> QNTVSHVSAACLFSEALHGIPFGVKVLKALAAANVSDASK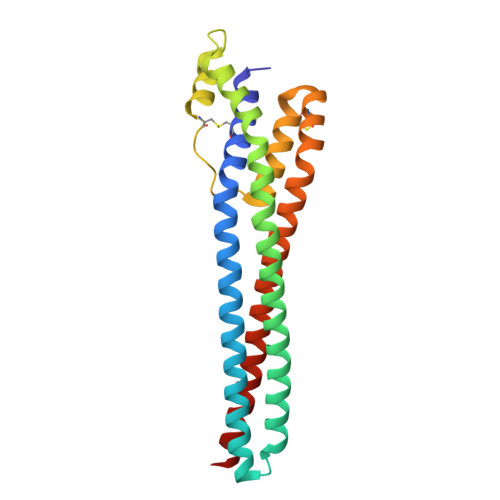AREGCQDAVRRAEDAFSSTPKVEEAVGRARAALKEAESAENAAKTALSDVEQYAANAPLLAAGKTAPIDDYLKSVAEDNSAASTARRIARGCSLPNRGVNSWVLKKAVEFGCEFFTGDICKILTDGMADLRAEYDQLEAAVRRASEARVAARAAESNARKAAEEAERTAA> MSKEIPTPYMWSYQPQMGLAAGASQDYSSRMNWLSAGPHMIGRVNGIRATRNQILLEQAALTSTPRSQLNPPNWPAVQVYQENPAPTTVLLPRDAEAEVQMTNSGAQLAGGSRHVRFRGRSSPYSPGPIKRLIIRGRGIQLNDEVVSSLTGLRPDGVFQLGGAGRSSFTPRQAYLTLQSSSSQPRSGGIGTLQFVEEFVPSVYFNPFS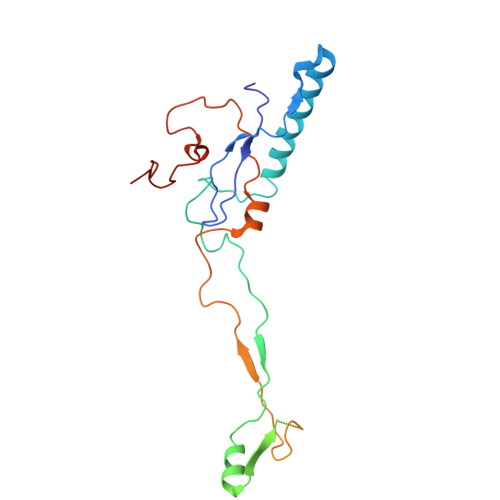GAPGLYPDDFIPNYDAVSESVDGYD> MQAAALLLLVLRAITSIEAAADDVNPDDNKEDFAVLCALAALANLQTTVPSIDTSGLAAYDNLQQLNLSLSSKEWKSLFNKAADSNGSPKQPPEGFQS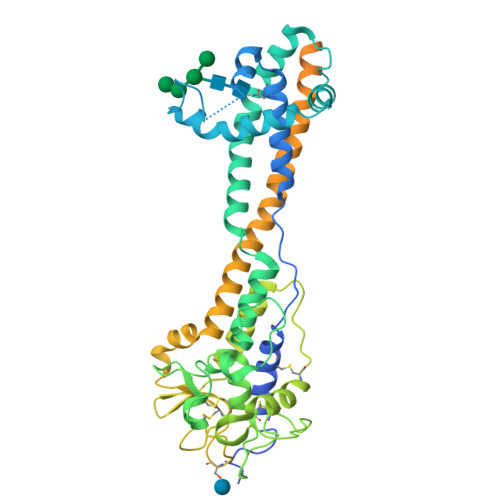DPTWRKQWPIWVTAAAALKAENKEAAVLARAGLTNAPEELRNRARLALIPLLAQAEQIRDRLSEIQKQNEDTTPTAIAKALNKAVYGQDKETGAVYNSADCFSGNVADSTQNSCKAGNQASKATTVAATIVCVCHKKNGGNDAANACGRLINHQSDAGANLATASSDFGDIIATCAARPPKPLTAAYLDSALAAVSARIRFKNGNGYLGKFKATGCTGAASEGLCVEYTALTAATMQNFYKIPWVKEISNVAEALKRTEKDAAESTLLSTWLKASENQGNSVAQKLIKVGDSKAVPPAQRQTQNKPGSNCNKNLKKSECKDSDGCKWNRTEETEGDFCKPKETGTENPAAGTGEGAAGANTETKKCSDKKTEGDCKDGCKWDGKECKDSSILATKKFALTVVSAAFVALLF N-benzylthioformamide 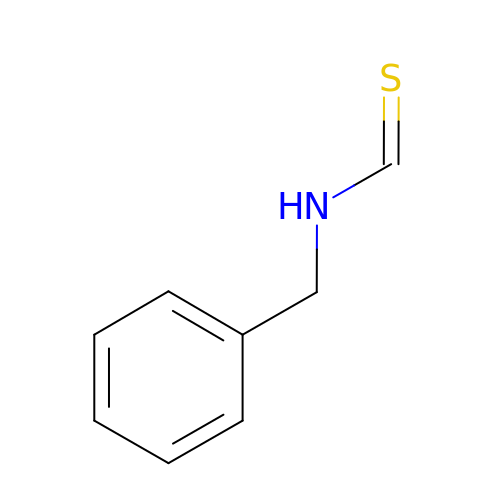| C8 H9 N S | QAADZYUXQLUXFX-UHFFFAOYSA-N>AMLIKPKRLQPGDIVATVSPSWGGAGDSEIRWRYEQGVKRLEEVFGLTVVPMPNSLKGSEFIYNNPQARAEDLMTAFQDTRVKAIIANIGGQDSIRLLPYIDFNAIRENPKIFMGYADVTISHLFCHKAGLSSFYGPAILTDFAENVEMDPYTVEMVNRTLFSNEMIGEIQPAPEWTSERLEWIEINKDTRRTMQQNNGYELLQGSTTVQGRLIGGCIEVLEFAKGTELWPEKKHWEDSILFFETSEDHPEPSYIKYWLRNYAAQGILQKAKGIIFGKP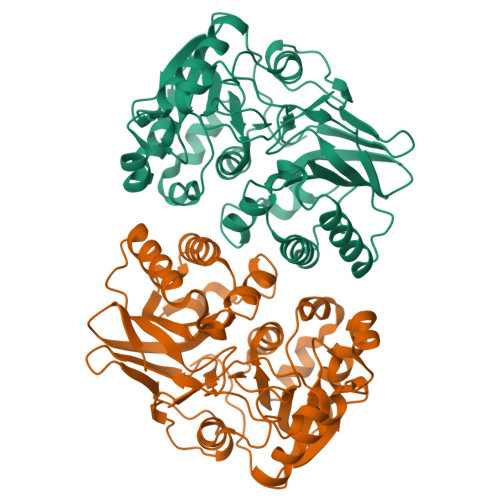KDEMYYEEYKHEILQVMKEHNLEDLPILYNLNFGHTEPKFILPYGSMAEIDCENGSFSILESGVE[4x]>[2x]MLPAVPPQQWALSAGNGSSEVEVVPFQEVWGRSYCRALERLVDVVSEYPSEVEHMFSPSCVSLLRCTGCCGDENLHCVPVETANVTMQLLKIRSGDRPSYVELTFSQHVRCECRPLRE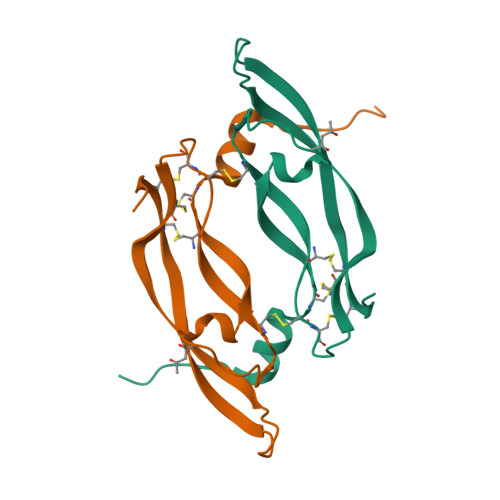KMKPERCGDAVPRR> MELSASATELLQDYMLTLRTKLSSQEIQQFAALLHEYRNGASIHEFCINLRQLYGDSRKFLLLGLRPFIPEKDSQHFENFLETIGVKDGRGII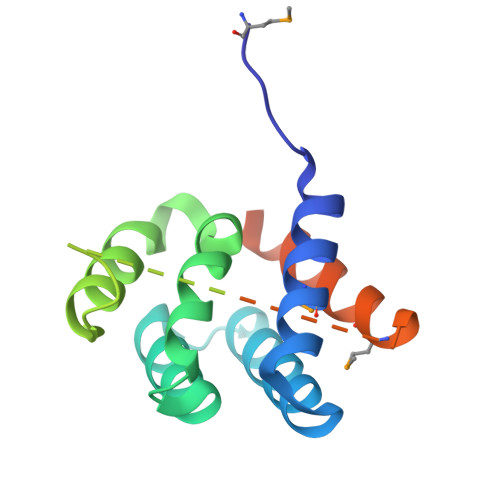TDSFGRHRRALSTTSSSTTNGNRATGSSDDRSAPSEGDEWDRMISDISSDIEALGCSMDQDSALEHHHHHH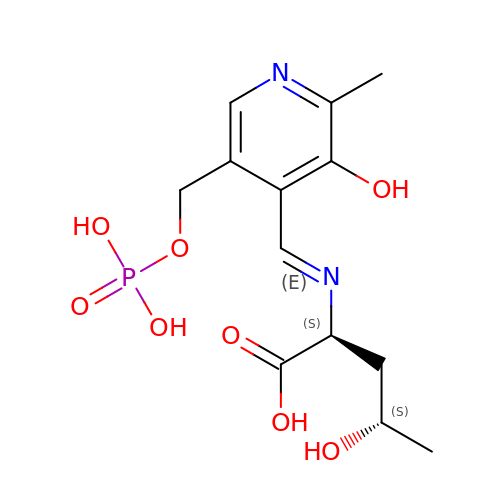N-(HYDROXY{3-HYDROXY-2-METHYL-5-[(PHOSPHONOOXY)METHYL]PYRIDIN-4-YL}METHYL)NORVALINE | C13 H19 N2 O8 P | XZPXXYMXESJHME-PMICCBOBSA-N>[2x]HRTIQLPGLINIAAFVPGLVTRDSEDLQRVTQASIAAGYSMIRIMPVSKDGSISDVKSLKVAQQNSKRGVYCDFNLSITATSDNANQISSVAGEVGSLFIPFNHLSDNISKVTQVEAHFDAWPKHK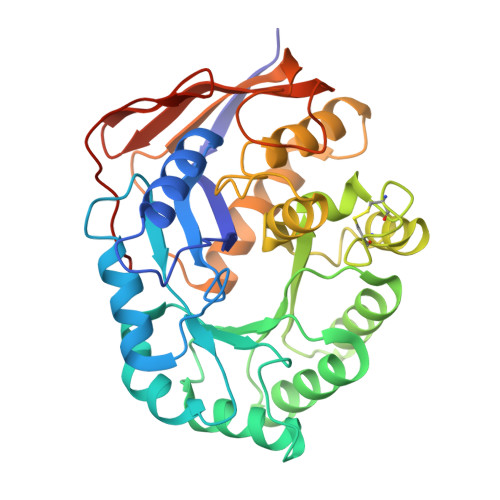PIITDARTTDLASILLLASLHNRRIHVSAVTTKDDIKLITLGKQKGLKVTCDVCVYSLFLSQKDCPGCHFLPTPEDQEALWEHLPIIDVFSIGSLPYQLAHFLKKEADVTVGIADALPLLLTAVVDGRLTVDYVKTRLHDNPKEIFELHDQVGATVEIELDRAFAVPTEGVWSPFAGKVLKGVVQRVTFQDQVACLDGVFQPIPPKGADMSTYGAL> MHHHHHHMVDEILKLKKEKGYIILAHNYQIPELQDIADFVGDSLQLARKAMELSEKKILFLGVDFMAELVKILNPDKKVIVPDRSATCPMANRLTPEIIREYREKFPDAPVVLYVNSTSECKTLADVICTSANAVEVVKKLDSSVVIFGPDRNLGEYVAEKTGKKVITIPENGHCPVHQFNAESIDAVRKKYPDAKVIVHPECPKPVRDKADYVGSTGQMEKIPERDPSRIFVIGTEIGMIHKLKKKFPDREFVPLEMAVCVNMK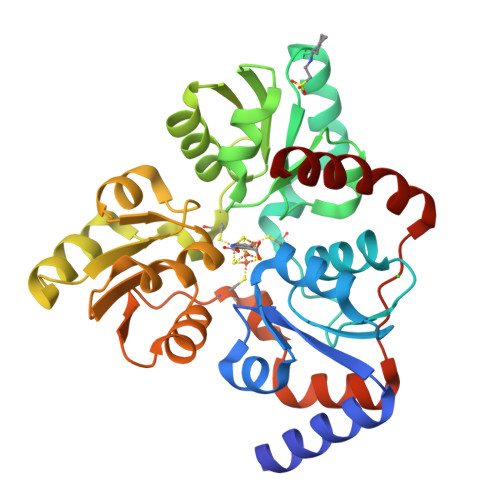KNTLENTLHALQTESFEVILPKEVIEKAKKPILRMFELMG> GPGSSRWSKDYDVCVCHSEEDLVAAQDLVSYLEGSTASLRCFLQLRDATPGGAIVSELCQALSSSHCRVLLITPGFLQDPWCKYQMLQALTEAPGAEGCTIPLLSGLSRAAYPPELRFM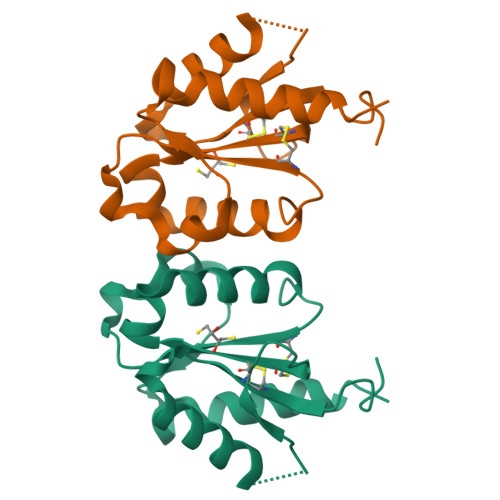YYVDGRGPDGGFRQVKEAVMRYLQTLS> DYKDDDDKMVVVTGREPDSRHSDGAMSSSEAEDDFLEPATPTATQAGHGLPLLPQEFPEVVPLNIGG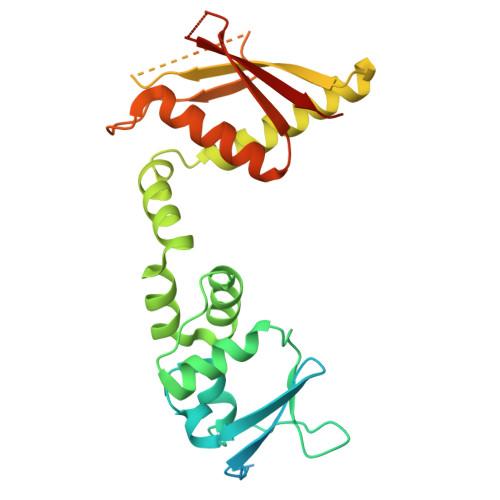AHFTTRLSTLRRYEDTMLAAMFSGRHYIPTDSEGRYFIDRDGTHFGDVLNFLRSGDLPPREHVRAVYKEAQYYAIGPLLEQLENMQPLKGEKVRQAFLGLMPYYKDHLERIVEIARLRAVQRKARFAKLKVCVFKEEMPITPYECPLLNSLRFERSESDGQLFEHHCEVDVSFGPWEAVADVYDLLHCLVTDLSAQGLTVDHQCIGVCDKHLVNHYYCKRPIYEFKITWW>[3x]SNASDWSLSQLFASLHE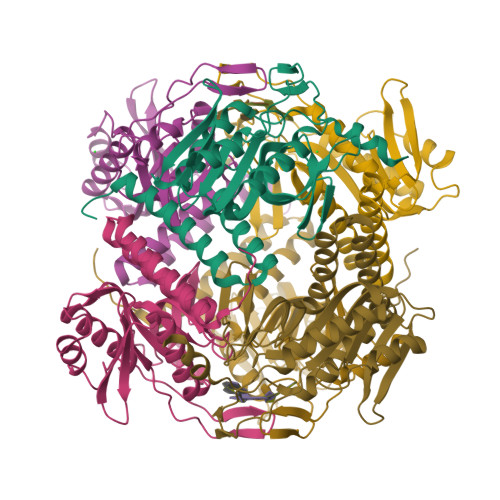DIQLRLGTARKAFQHPGAKGDASEGVWIEMLDTYLPKRYQAANAFVVDSLGNFSDQINVVVFDRQYSPFIFKFNEQIIVPAESVYAVFEAKQSASADLVAYAQRKVASVRRLHRTSLPIPHAGGTYPAKPLIPILGGLLTFESDWSPALGMSFDKALNGDLSDGRLDMGCVASHGHFYFNNIDSKFNFEHGNKPATAFLFRLIAQLQFSGTVPMIDIDAYGKWLAN>AYKLIKMAGGNSAIQTYAREDKTTQTLSTQKTISVLRNGSTSTRIIKVHINSTAPVTINTCDPTKCGPTVPMGVSFKSSMPEDADPAEVLKAAKAALALFEA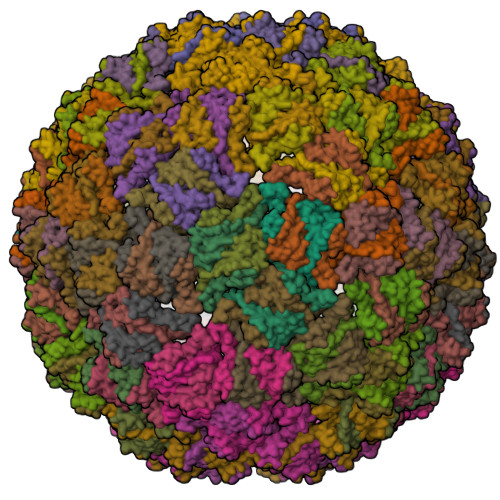NLNSAFNKNVDEISVA[60x]>[9x]MDWHIAKHYDDILYYKAGGIAKIVINRPHKR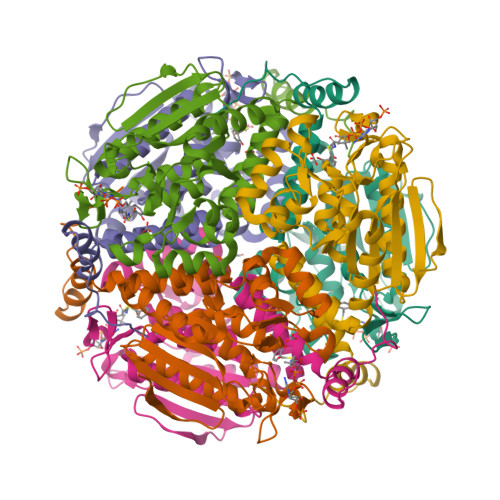NAFRPQTVFELYDAFCNAREDNRIGVVLLTGAGPHSDGKYAFCSGGDQSVRGEGGYIDDQGTPRLNVLDLQRLIRSMPKVVIALVAGYAIGGGHVLHLVCDLTIAADNAIFGQTGPKVGSFDGGFGSSYLARIVGQKKAREIWYLCRQYSAQEAERMGMVNTVVPVDRLEEEGIQWAKEILSKSPLAIRCLKAAFNADCDGQAGLQELAGNATLLYYMTEEGSEGKQAFLEKRPPDFSQYPWLP>[2x]GDEKQFQIEKWQIARCNKSKPQKFINDLMQVLYTNEYMATHSLTGAKSSTSRDKAVKPAMNQNEVQEIIGVTKQLFPNTDDVSIRRMIGQKLNNCTKKPNLSK

pmcThe BEN (BANP, E5R, and NAC1) domain is a ∼100-residue protein domain found in metazoans and viruses, but missing in nematodes and urochordates. There are nine BEN domain–containing transcription factors in the human genome, i.e., BANP, BEND2-7, and NAC1/2. The BEN domain-containing transcription factors regulate transcription by recruiting chromatin-modifying factors to specific chromatin regions via their DNA-binding BEN domains. Further structural analysis revealed that although all these BEN domains bind their target DNAs mainly through the insertion of the C-terminal α5 helix into the major groove of DNA, the residues of the α5 helices involved in the base interactions vary from one to another, explaining why they exhibit distinct DNA sequence preference.

To further investigate the role of cytosine methylation in BEN domain binding, we successfully obtained the structures of the BEND6 BEN domain in complexes with the CGCG motif and CGmCG motif containing DNAs, respectively. Our binding results also revealed that the BEN domain of BEND6 exhibited comparable binding affinities to the methylated and unmethylated CGCG motif DNA sequences with Kd of ∼39 μM and ∼33 μM, respectively. In the BEND6-CGmCG structure, two BEND6 BEN domain molecules bound to a DNA duplex in an asymmetric unit. The two BEND6 molecules could be superimposed very well, and they bound to the DNA in roughly the same binding mode. For instance, both BEND6 molecules used N262, N261, and S217 to make hydrogen-bonding interactions with the bases of C3, G5’, and G8 of the DNA, respectively, although N262 of the BEND6 molecule 1 formed a water-mediated interaction with the base of C3, while N262 of the BEND6 molecule 2 formed a direct interaction with the base of C3. Moreover, we found that the binding mode of the CGmCG DNA to the BEND6 BEN domain was very similar to that observed in the BEND6-CGCG DNA complex. Similar to the BEND6-CGCG DNA structure, R254 interacted with the base of G7’ in one molecule and interacted with the DNA backbone in the other molecule. In both structures, the last six amino acid residues (K266 to K271) after the helix α5 are disordered.> MYDFTNCDFEKIKAAYLSTISKDLITYMSGTKSTEFNNTVSCSNRPHCLTEIQSLTFNPTAGCASLAKEMFAMKTKAALAIWCPGYSETQINATQAMKKRRKRKVTTNKCLEQVSQLQGLWRRFNRPL;> CHWLENCW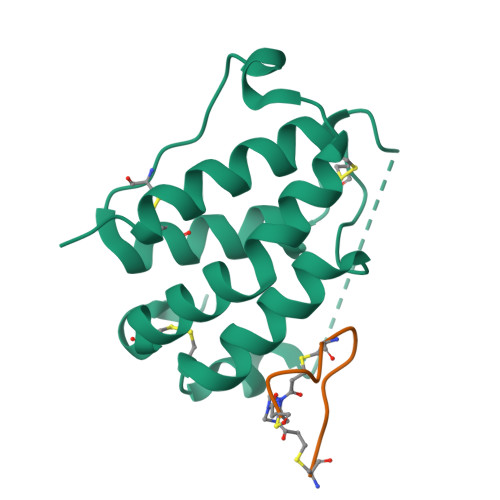RGFC> GSKQKEAIKVYLELLEVHSRVLKALIEQIKLFIELIKRPDEDLADKVRKS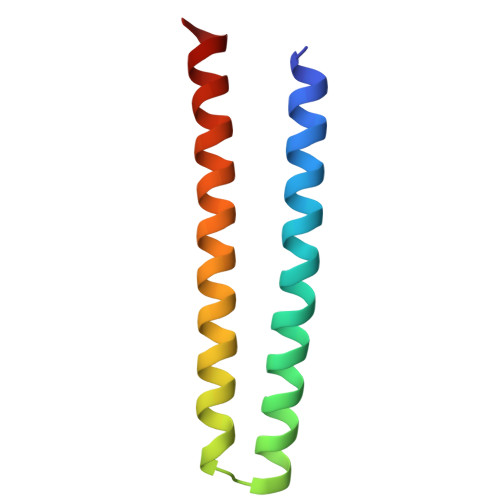SEELKKIIKEVEKILRKVDDILYKVKS>GSHMASFLKRYTSNTYSKDEEKLIQSVSKAVQYMAKRRIGALIVFEKETGLQDYIETGIAMDSNISQELLICVFIPNCPLHDGAMIIQGTKIAAAASYLPLSDSPKISKSLGTRHRAAVGISEVSDAFTVIVSEETGDISVTFDGKLRRDISNEIFEELLAEHWFGTRFQKKGVK[2x]

In the human pathogen Staphylococcus aureus, c-di-AMP is produced by the di-adenylate cyclase enzyme DacA, which is thought to form a complex and be regulated by YbbR and GlmM, two other conserved proteins. GlmM codes for the essential phosphoglucosamine mutase enzyme, required for the conversion of glucosamine-6-phosphate to the early peptidoglycan synthesis precursor glucosamine-1-phosphate. We determined the atomic structures of the S. aureus DacA and GlmM enzymes and show that GlmM readily binds to DacA in vitro and blocks its activity by masking its active site. Specifically, our data suggest that GlmM blocks access to the active site of DacA and in this manner prevents the formation of catalytically active head-to-head DacA oligomers.

Two key interacting residues in the dimer interface are amino acids N166 and T172. To potentially disrupt this interaction, we mutated these two residues to lysines, yielding variant DacACD-K. To “lock” the dimer conformation, we also mutated these residues to cysteines (DacACD-C variant) to facilitate the formation of disulfide bonds between the two protomers. To further assess if the DacACD-C variant could form disulfide-bridge locked dimers, the purified protein was crystallized and its structure determined. The protein crystallized in the same dimeric conformation as the DacACD protein and electron densities consistent with the formation of two disulfide bonds were observed for the DacACD-C variant, which were absent in the DacACD protein. The WT DacACD and DacACD-C variant had similar elution profiles and eluted at a retention volume as expected for a DacACD dimer. The DacACD-C variant displayed very similar activity to the WT DacACD protein, suggesting that locking the dimer through two disulfide bridges does not influence the activity of the enzyme. The melting curves for the DacACD and DacACD-C proteins were sigmoidal, which is typical for well-folded proteins. Taken together, these data show that WT DacACD and the ‘locked-dimer’ DacACD-C variant show similar enzymatic activities, suggesting that the stable dimer we observed in our crystal structures will likely transiently interact with other dimers to form higher oligomers for catalysis and c-di-AMP product formation.>CGCGCG[6x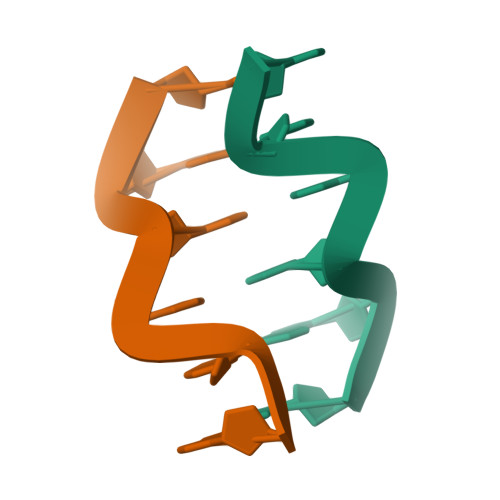]>MHHHHHHGSLLPATHELHIFGSINSLEFDLVGRGTGNPKEGYEELHLKSTKSALQFSPWILVPQIGYGFYQYLPFPDGAMSPFQAAMNDGSGYQVHRTMQFEDGATLTGIYRYTYEGTHIKGEFQVIGTGFPADGPVMTNSLTAADWCVTKIVYPNENTIIDKFDWTYTTTSGKRYQSNVRSNFTFAKPIAA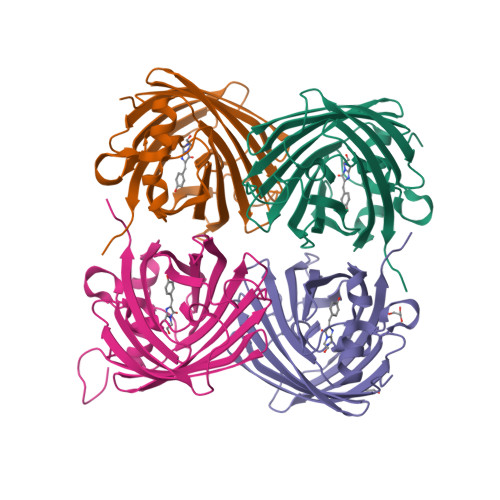NILQKQPMFVFRKTELKHSKTELNFKEWQTAFSDVM[4x]> ADIGSNIFYAGDATKSNYFRIPSLLALDSGTVIAAADARYGGTHDAKSKINTAFAKSTDGGKTWGQPTLPLKFDDYVAKNIDWPRDSVGKNVQIQGSASYIDPVLLEDKETHRVFLFADMMPAGIGSSNASVGSGFKEVDGKKYLKLHWKDDAAGTYDYSVRENGTIYNDTTNSATEYSVDGEYNLYKNGNAMLCKQYDYNFEGTKLLETQTDTDVNMNVFYKDADFKVFPTTYLAMKYSDDEGETWSDLQIVSTFKPEESKFLVLGPGVGKQIANGEHAGRLIVPLYSKSSAELGFMYSDDHGNNWTYVEADQNTGGATAEAQIVEMPDGSLKTYLRTGSGYIAQVMSTDGGETWSERVPLTEIATTGYGTQLSVINYSQPVDGKPAILLSAPNATNGRKNGKIWIGLISETGNSGKDKYSVDWKYCYSVDTPQMGYSYSCLTELPDGEIGLLYEKYDSWSRNELHLKNILKYERFNIDELKVQP

Here we functionally and structurally characterize R. gnavus ATCC 29149 sialidase (RgNanH), demonstrating that the enzyme is an intramolecular trans-sialidase (IT-sialidase) producing 2,7-anhydro-Neu5Ac selectively from α2-3-linked sialic acid substrates, the first one reported in a gut commensal microbe suggesting an unprecedented mechanism underpinning adaptation of gut bacteria to the sialylated-rich mucosal environment. RgNanH catalytic domain (residues 243–723) was heterologously expressed and purified, and the crystal structure of the N-domain with the inserted I-domain (NI-domain) was solved to a maximum resolution of 1.71 Å. RgNanH active site presents the classical features of bacterial sialidases, shared by hydrolytic and trans-sialidases. These include an arginine triad formed by Arg257, Arg637 and Arg575; a catalytic pair formed by Glu559 and Tyr677; a general acid base, Asp282; and a pocket to accommodate the N-acetyl group.

Complexes with Neu5Ac2en, OC and siastatin B, bound in the active site, were solved to 2.00, 2.01 and 1.94 Å, respectively. Our crystal structures of RgNanH inhibitor complexes, including the first published structure of a complex between siastatin B and a sialidase, provide a structural explanation for the differences in inhibition between the chemical inhibitors tested. Siastatin B (IC50 of ∼5 μM) was the most potent inhibitor tested. Siastatin B is based on an iminosugar scaffold with carboxylic acid, hydroxyl and N-acetyl functional groups at equivalent positions to Neu5Ac, an additional hydroxyl group is present at position 3. The siastatin B inhibitor bound to the active site in a chair conformation. Like Neu5Ac2en, the carboxylic acid group of siastatin B interacts with the arginine triad, and the O4 hydroxyl with Arg276 and Asp339. Furthermore, the axial C3 hydroxyl of siastatin B formed hydrogen bonds to Asp282 and Arg257 of the arginine triad. Furthermore, in comparison with Neu5Ac2en and OC, siastatin B makes a more extensive hydrogen-bonding network underneath the ligand via the buried water. Finally, although both Neu5Ac2en and siastatin B form hydrogen bonds to Asp282 (Neu5Ac2en via the glycerol group), siastatin B achieves such interaction without paying the entropic penalty required to avoid a steric clash between the glycerol group and Thr557.>GSSMKISRGLLKTILEAAKSAHPDEFIALLSGSKDVMDELIFLPFVSGSV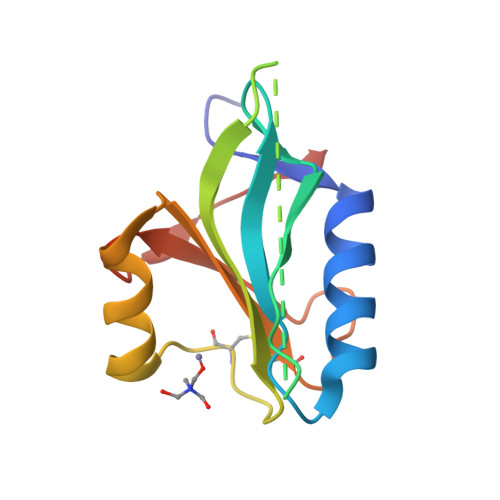SAVIHLDMLPIGMKVFGTVHSHPSPSCRPSEEDLSLFTRFGKYHIIVCYPYDENSWKCYNRKGEEVELEVVEKD[4x]> GSHMSELSEIDSVAGVTIYSVDGEPKSFVYKAGFAIDADGAPNAYAPNNGGTDFTANGGDDQGGDWWGGPVDAEGYPIKQKIFDPFPGYYVSATAHFNPAYSEDSPYRYIDSNSIPFIVLPGNHSNGAKLGDVALVYNEK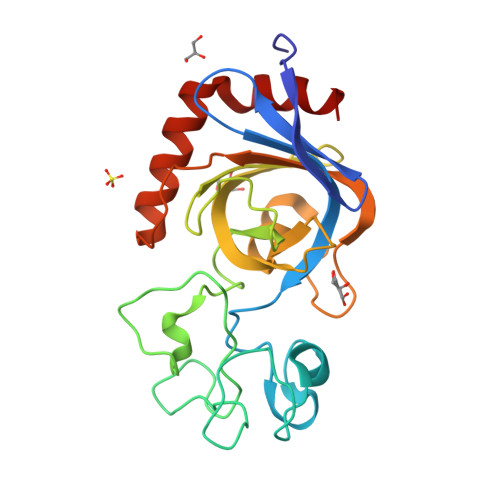TGDNCYAIYGDVGPSSKIGEGSVRLAQALKIDDNPKAGGTESRIVVTLVFPGSVGKWETPKRWFSHANQLTKAWGGLSRLKTLSDQL4-(2-chlorophenyl)-3-hydroxy-7,7-dimethyl-2-phenyl-2,6,7,8-tetrahydro-5H-pyrazolo[3,4-b]quinolin-5-one | C24 H20 Cl N3 O2 | 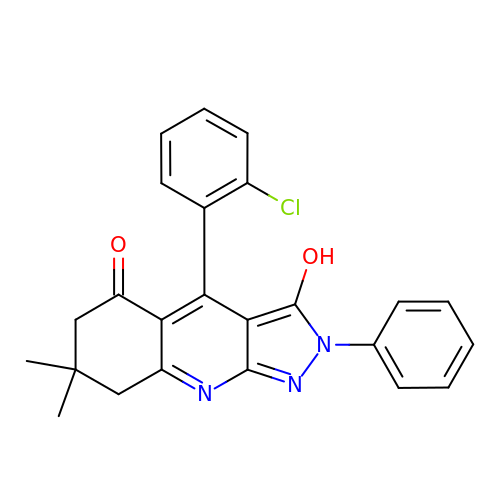RZRIAROHONSNNR-UHFFFAOYSA-N>[2x]TYLDRLALRYDREGEPSQLAAVDIFVSTVDPLKEPPLVTANTVLSILAVDYPVDKVSCYVSDDGAAMLSFESLAETSEFARKWVPFCKKYSIEPRAPEWYFAAKIDYLKDKVQTSFVKDRRAMKREYEEFKIRINALVSKALKCPEE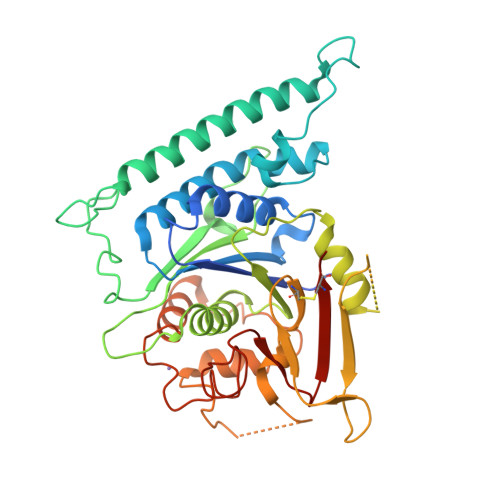GWVMQDGTPWPGNNTRDHPGMIQVFLGQNGGLDAEGNELPRLVYVSREKRPGFQHHKKAGAMNALVRVSAVLTNGPFILNLDCDHYINNSKALREAMCFLMDPNLGKQVCYVQFPQRFDGIDKNDRYANRNTVFFDINLRGLDGIQGPVYVGTGCVFNRTALYGYEPGSGSGSLEKRFGQSAVFVASTLMENGGVPPSATPENLLKEAIHVISCGYEDKSDWGMEIGWIYGSVTEDILTGFKMHARGWRSIYCMPKLPAFKGS> SNAMLTLLPAV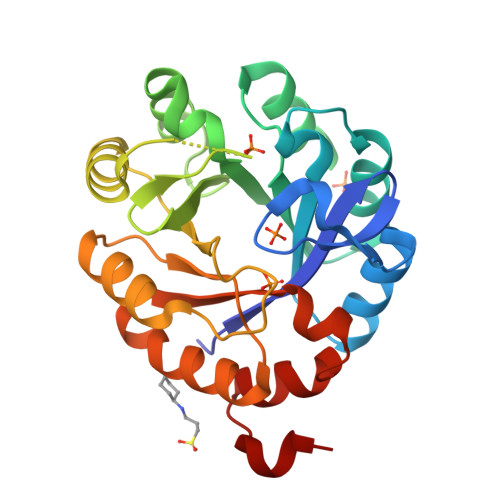DVADGKAVRLLQGEAGSETDYGSPIEAARDWVEAGAEWIHLVDLDAAFGRGSNAPLLERIVGEVGIKVELSGGIRDDASLTRALKAGAARVNLGTAALEDPQWTARVIAEHGEKIAVGLDVRGTTLAARGWTKEGGDLWQTLDRLNEAGCRRYVVTDVTKDGTLTGPNTELLRQVAARTSAPVVASGGISSLEDIAALARLVPQGVDSAIVGKALYNGNFTLPQALAVAGGAAVQDVQA>[2x]ACYCRIPACIAGERRYGTCIYQG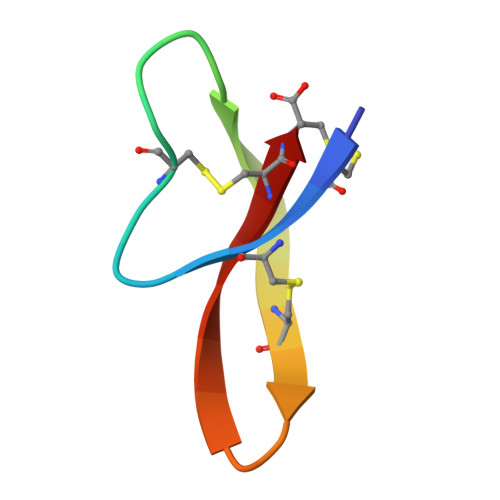ALWAFCC Recently, the YEATS (YAF9, ENL, AF9, TAF14, SAS5) domains were identified as “readers” of lysine acylation, including acetylation and crotonylation. Unlike the bromodomains with end-closed binding cavities, the YEATS domain adopts an end-open aromatic “sandwich” cage to recognize histone lysine acylation. The AF9 YEATS domain adopted an immunoglobin fold that consisted of a two-layer β sandwich between eight antiparallel β strands. The AF9/ENL YEATS domains recognize acylated histones to recruit the super elongation complex and, in turn, DOT1L on active chromatin.

Herein, we identified four small-molecule hits against the AF9 YEATS domain using NMR fragment-based screening. The crystal structure of the AF9 YEATS domain in complex with hit 2 was hence solved to depict their interaction mode. The highly conserved residues F28, H56, S58, F59, Y78, and F81 together formed a serine-lined aromatic cage for acyl-lysine recognition, where hit 2 was embedded with a clearly visible electron density. The benzyl moiety of hit 2 interacted with H56 through π-π stacking. The amide nitrogen and ether oxygen of hit 2 participated in the formation of hydrogen bonds with the side-chain hydroxyl of S58, while the carbonyl group of hit 2 formed a hydrogen bond with the backbone amide of Y78. Furthermore, this carbonyl group also participated in the water-mediated hydrogen bonds with W32 and A79. The structure of AF9 YEATS in complex with hit 2 indicated the feasibility to improve ligand potency. Furthermore, superimposition of the crystal structures of AF9 YEATS in complex with hit 2 or H3K9cr peptide suggested that the chlorine group of hit 2 may be substituted. As the crystal structure also revealed that the methoxyl group of hit 2 pointed toward the unoccupied groove surrounded by residues F28, P60, and E75, we substituted the methyl group with a benzyl or phenyl group (compounds 10 and 11). The binding affinity of hit 2 was then determined by best fitting the dose-dependent CSPs of these residues at 0.07 ± 0.01 mM (fitting error was used henceforth unless specifically annotated).

>MASSCAVQVKLELGHRAQVRKKPTVEGFTHDWMVFVRGPEHSNIQHFVEKVVFHLHESFPRPKRVCKDPPYKVEESGYAGFILPIEVYFKNKEEPRKVRFDYDLFLHLEGHPPVNHLRCEKLTFNNPTEDFRRKLLKA[2x]3-AMINOPYRIDINE 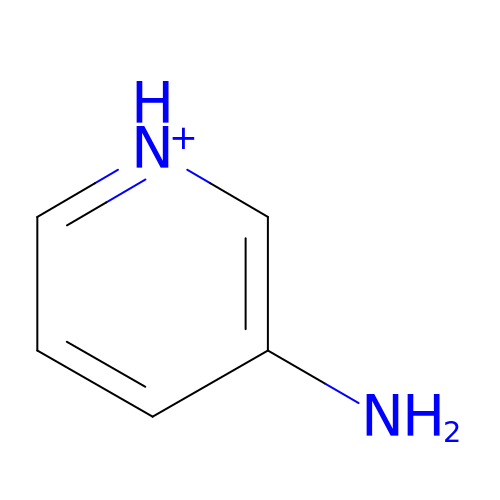| C5 H7 N2 | CUYKNJBYIJFRCU-UHFFFAOYSA-O> VSLPRMVYPQPKVLTPCRKDVLVVTPWLAPIVWEGTFNIDILNEQFRLQNTTIGLTVFAIKKYVAFLKLFLETAEKHFMVGHRVHYYVFTDQPAAVPRVTLGTGRQLSVLEVRAYKRWQDVSMRRMEMISDFCERRFLSEVDYLVCVDVDMEFRDHVGVEILTPLFGTLHPSFYGSSREAFTYERRPQSQAYIPKDEGDFYYMGAFFGGSVQEVQRLTR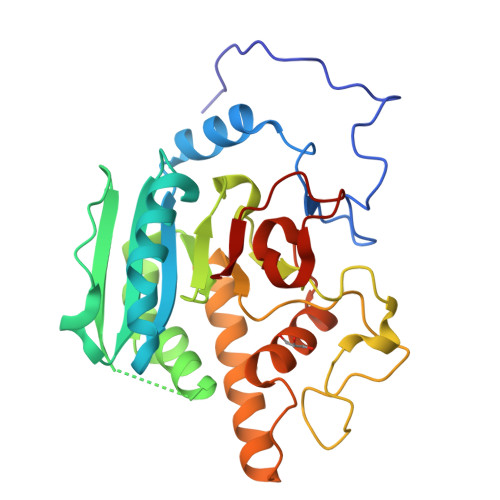ACHQAMMVDQANGIEAVWHLESHLNKYLLRHKPTKVLSPEYLWDQQLLGWPAVLRKLRFTAVP>[2x]MVDSVYRTRSLGVAAEGLPDQYADGEAARVWQLYIGDTRSRTAEYKAWLLGLLRQHGCQRVLDVACGTGVDSIMLVEEGFSVTSVDASDKMLKYALKERWNRRHEPAFDKWVIEEANWMTLDKDVPQSAEGGFDAVICLGNSFAHLPDCKGDQSEHRLALKNIASMVRAGGLLVIDNRNYDHILSTGCAPPGKNIYYKSDLTKDVTTSVLIVNNKAHMVTLDYTVQVPGAGQDGSPGLSKFRL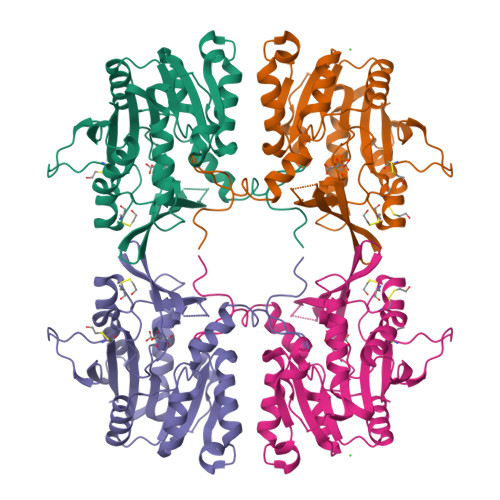SYYPHCLASFTELLQAAFGGKCQHSVLGDFKPYKPGQTYIPCYFIHVLKRTD> SMLKYSTNMLELAMPKINKIVNGTDLTPHYLSEPNKEFKIYRYNNEVYAVRFENDEPMDYVLMWKSHKSEHTQNSEMIKNTEEDYKELGKGEQGTVYEKTEDKAMKVSRGRHPREFYEEINLHIIEQQFFLKYHGIQEHFVLGLWNIKNEENVYFYMPKINAIPINKKIDQPKIEEF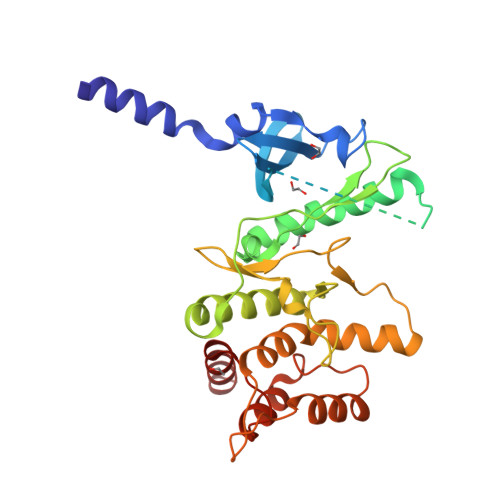VLALKELNDAGYWHPDLANNPYHISPQNLIATEEMVKTIDLDGGFRYDKGRVDELSRKSLVYGKDQWLYVYNFIYPPTDEEDHRIDWRVPIEKWYENNRDESLSDNPHTLLRFYHEGLISLPKKLAHDLHETILEEL> GAQSCVWYGECGIAYGDKRYNCEYSGPPKPLPKDGYDLVQELCPGFFFGQVSLCCDVRQLQTLKDNLQLPLQFLSRCPSCFYNLLNLFCELTCSPRQSQFLQVTATEDYVDPVTNQTKTNVKELQYYVGQSFANAMYNACRDVEAPSSNDKALGLLCGKDADACQATNWIEYMFNKDNGQAPF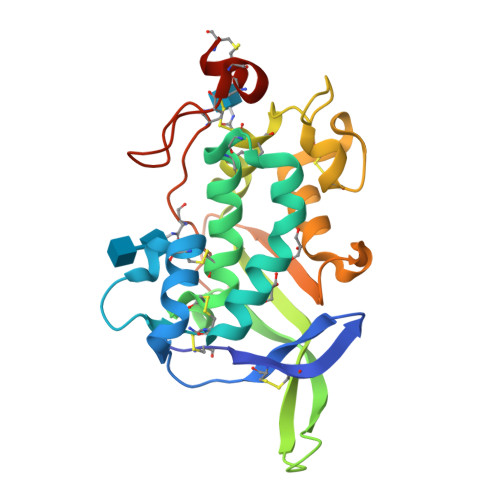TITPVFSDFPVHGMEPMNNATKGCDESVDEVTAPCSCQDCSIVCGPKPQ>GSTGSMTIGIDKISFFVPPYYIDMTALAEARNVDPGKFHIGIGQDQMAVNPISQDIVTFAANAAEAILTKEDKEAIDMVIVGTESSIDESKAAAVVLHRLMGIQPFARSFEIKEACYGATAGLQLAKNHVALHPDKKVLVVAADIAKYGLNSGGEPTQGAGAVAMLVSSEPRILALKEDNVMLTQDIYDFWRPTGHPYPMVD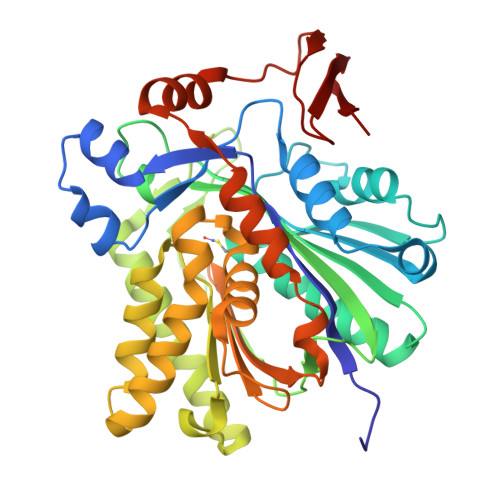GPLSNETYIQSFAQVWDEHKKRTGLDFADYDALAFHIPYTKMGKKALLAKISDQTEAEQERILARYEESIIYSRRVGNLYTGSLYLGLISLLENATTLTAGNQIGLFSYGSGAVAEFFTGELVAGYQNHLQKETHLALLDNRTELSIAEYEAMFAETLDTDIDQTLEDELKYSISAINNTVRSYRN[4x]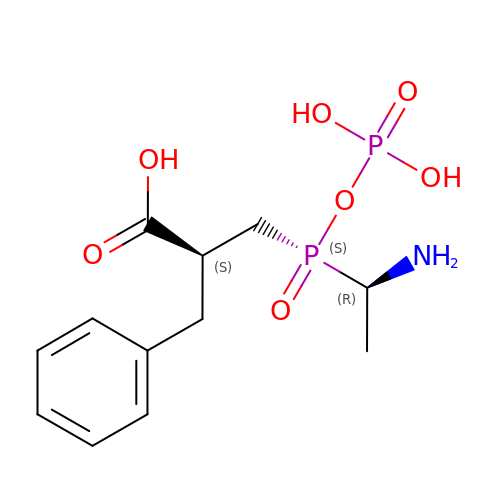(2S)-3-[(S)-[(1R)-1-aminoethyl](phosphonooxy)phosphoryl]-2-benzylpropanoic acid | C12 H19 N O7 P2 | KXASHFLSUHEZCK-UODZXCQVSA-N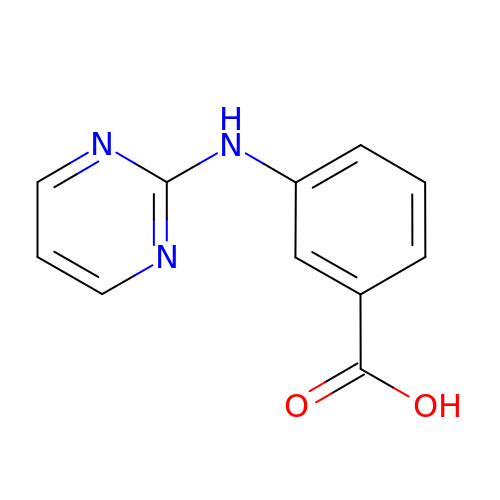3-[(pyrimidin-2-yl)amino]benzoic acid | C11 H9 N3 O2 | JCCQTGJTDPBYJP-UHFFFAOYSA-N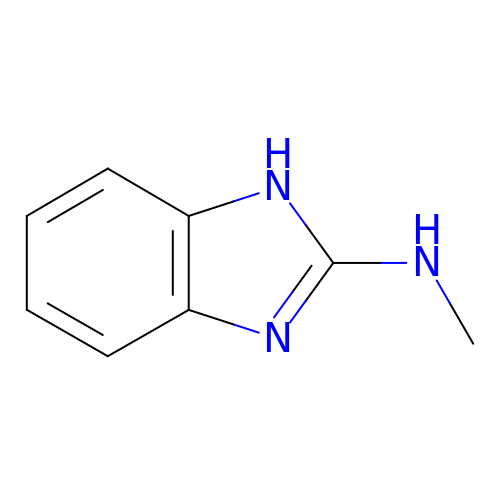N-methyl-1H-benzimidazol-2-amine | C8 H9 N3 | ALBBQFWHUCTZFM-UHFFFAOYSA-N>GPAVPRMDTTIDGFADSYEISSTSFVATDNTDSSIVYLAAEQVLTGPDVSALQLLSNSFESVFDSPDDFYSDAKLVLSDGREVSFHRCVLSARSSFFKSALAAAKKEKDSNNTAAVKLELKEIAKDYEVGFDSVVTVLAYVYSSRVRPPPKGVSECADENCCHVACRPAVDFMLEVLYLAFIFKIPELITLYQRHLLDVVDKVVIEDTLVILKLANICGKACMKLLDRCKEIIVKSNVDMVSLEKSLPEELVKEIIDRRKELGLEVPKVKKHVSNVHKALDSDDIELVKLLLKEDHTNLDDACALHFAVAYCNVKTATDLLKLDLADVNHRNPRGYTVLHVAAMRKEPQLILSLLEKGASASEATLEGRTALMIAKQATMAVECNNIPEQCKHSLKGRLCVEILEQEDKREQIPRDVPPSFAVAADELKMTLLDLENRVALAQRLFPTEAQAAMEIAEMKGTCEFIVTSLEPDRLTGTKRTSPGVKIAPFRILEEHQSRLKALSKTVELGKRFFPRCSAVLDQIMNCEDLTQLACGEDDTAEKRLQKKQRYMEIQETLKKAFSEDNLELGNSSLTDSTSSTSKSTGGKRSNRKLSHRRRGGWSHPQFER[2x];>[2x]GPANNDQDEDRINDKMKRRLAQNREAARKSRLRKKAHVQQLEESRLKLSQLEQELVRARQQGLCVRNSSDTSYLGPAGNMNSGIAAFEMEYTHWLEEQNRRVSEIRTALQAHIGDIELKMLVDSCLNHYANLFRMKADAAKADVFFLMSGMWRTSTERFFQWIGGFRPSELLNVVMPYVEPLTDQQLLEVRNLQQSSQQAEEALSQGLDKLQQGLVESIAIQIKVVESVNHGAPMASAMENLQALESFVNQADHLRQQT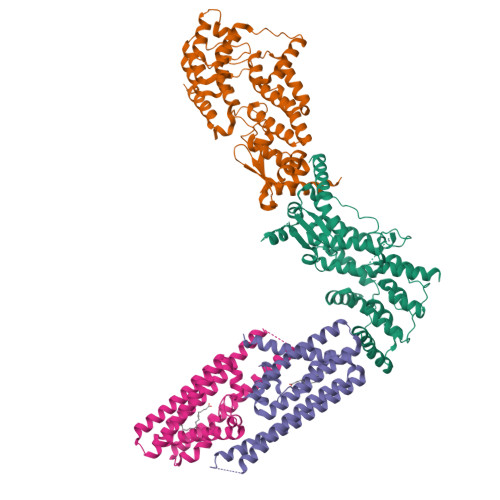LQQMSKILTTRQAARGLLALGEYFHRLRALSSLWAARPREHTGGDYKDDDDKSSGYPYDVPDYA> MSSYNSAIDQKTPSIKVLDNRKLNVRTLEYLRTQADENSDELITFYEFNIPGFQVKSTDPRKNKNQSGPNFIRVFNLAGQVLREESVDAGRTITLNDIESRPVLIINATGVRQNHRYEDNTLPGRLLAITEQVQAGEKTTERLIWAGNTPQEKDYNLAGQCVRHYDTAGLTQLNSLSLAGVVLSQSQQLLVDDKNADWTGEDQSLWQQKLSSDVYTTQNKADATGALLTQTDAKGNIQRLAYDVAGQLKGCWLTLKGQAEQVIIKSLTYSAAGQKLREEHGNGVITEYSYEPETQRLIGIATRRPSDAKVLQDLRYQYDPVGNVINIRNDAEATRFWRNQKVVPENSYTYDSLYQLISATGREMANIGQQNNQLPSPALPSDNNTYTNYTRSYSYDHSGNLTQIRHSSPATQNNYTVAITLSNRSNRGVLSTLTTDPNQVDTLFDAGGHQTSLLPGQTLIWTPRGELKQVNNGPGNEWYRYDSNGMRQLKVSEQPTQNTTQQQRVIYLPGLELRTTQSNATTTEELHVITLGEAGRAQVRVLHWESGKPEDVNNNQLRYSYDNLIGSSQLELDNQGQIISEEEYYPFGGTALWAANSQTEASYK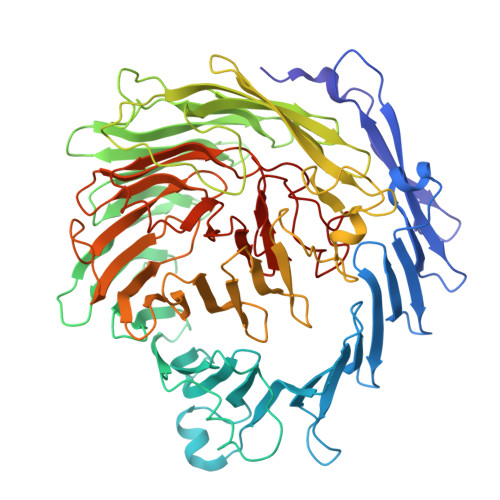TIRYSGKERDATGLYYYGYRYYQPWAGRWLSADPAGTIDGLNLYRMVRNNPVSLQDENGL> APYASLTEIEHLVQSVCKSYRETCQLRLEDLLRQRSNIFSREEVTGYQRKSMWEMWERCAHHLTEAIQYVVEFAKRLSGFMELCQNDQIVLLKAGAMEVVLVRMCRAYNADNRTVFFEGKYGGMELFRALGCSELISSIFDFSHSLSALHFSEDEIALYTALVLINAHRPGLQEKRKVEQLQY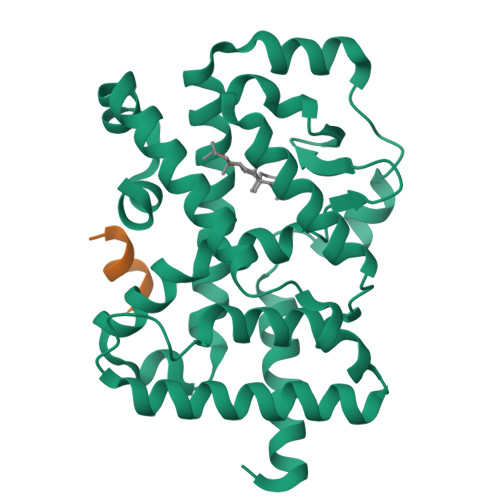NLELAFHHHLCKTHRQSILAKLPPKGKLRSLCSQHVERLQIFQHLHPIVVQAAFPPLYKELFS;> KHKILHRLLQDSS> GAQVTRQQTGTHENANIATNGSHITYNQINFYK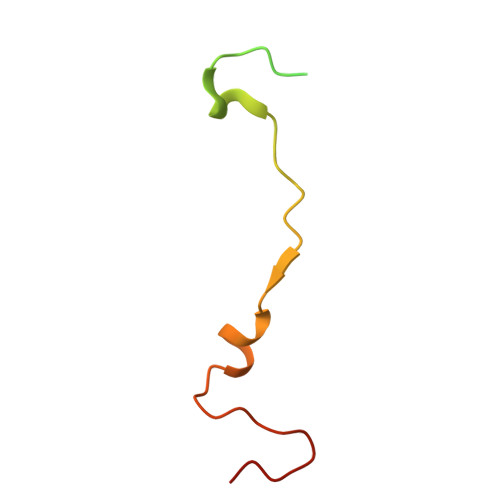DSYAASASKQDFSQDPSKFTEPVVEGLKAGAPVLK> MAASCVLLHTGQKMPLIGLGTWKSEPGQVKAAIKYALTVGYRHIDCAAIY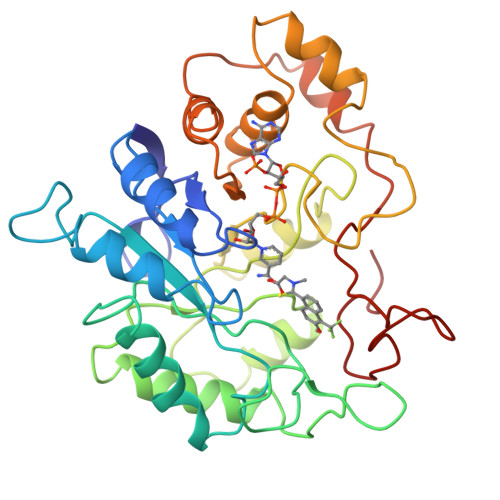GNELEIGEALTETVGPGKAVPREELFVTSKLWNTKHHPEDVEPALRKTLADLQLEYLDLYLMHWPYAFERGDNPFPKNADGTIRYDATHYKDTWKALEALVAKGLVRALGLSNFSSRQIDDVLSVASVRPAVLQVECHPYLAQNELIAHCQARGLEVTAYSPLGSSDRAWRDPNEPVLLEEPVVQALAEKYNRSPAQILLRWQVQRKVICIPKSVTPSRIPQNIQVFDFTFSPEEMKQLDALNKNLRFIVPMLTVDGKRVPRDAGHPLYPFNDPY Membrane-bound pyrophosphatases (M-PPases) are enzymes that couple the synthesis or hydrolysis of pyrophosphate (PPi) to the vectorial transport of protons and/or sodium ions. In addition, M-PPases can be divided into seven functional classes on the basis of their monovalent cation binding (K+-dependent and K+-independent enzymes) and pumping specificity (H+-pumps (H+-PPases), Na+-pumps (Na+-PPases) and H+ and Na+ co-pumps (Na+/H+-PPases)) and on the placement of a ‘semi-conserved glutamate' essential for pumping activity. So far, the structures of two M-PPases have been solved in three different states: TmPPase in resting and product-bound states (TmPPase:Ca:Mg and TmPPase:Pi2, respectively)11 and VrPPase in a substrate-analogue imidodiphosphate (IDP)-bound state (VrPPase:IDP)12. These structures have shown that M-PPases are homodimers, with each protomer having 16 transmembrane helices (TMHs) and a vertically arranged, continuous active site structure with four distinctive parts: ‘hydrolytic centre', ‘coupling funnel', ‘ion gate' and ‘exit channel'3. In this article we present three structures: the Na+-pumping TmPPase with IDP and Na+ bound (TmPPase:IDP) at 3.5 Å resolution, the H+-pumping VrPPase with one phosphate bound (VrPPase:Pi) at 3.5 Å resolution, and the newly refined structure of TmPPase with the phosphate analogue, WO4 bound, at 4 Å resolution (TmPPase:WO4).

In TmPPase:IDP, an Mg5IDP-complex was fit into the positive Fo–Fc density in the hydrolytic centre and then refined. The coordination of Mg2+ and IDP is almost identical to that seen in VrPPase:IDP12, even though the two enzymes pump different ions. Positive Fo–Fc density was seen in TmPPase:IDP between residues D6.50, E6.53, S6.54 and D16.46. A sodium ion was therefore refined into this density. The resulting bond distances were between 2.39–2.49 Å (mean: 2.43 Å) and the site was penta-coordinated (by the carboxylate groups of D6.50, E6.53 and D16.46, the Oγ of S6.54 and the main-chain carbonyl of D6.50)18. All of these results indicate that the density is most likely a bound Na+ and not a water molecule. Close to this, K16.50, which forms an ion-triplet in the resting-state TmPPase structure with D6.50 and E6.53, adopts a different orientation and the K16.50 Nζ is disordered. In TmPPase, sodium binding is facilitated by the inward motion of D16.46 into the sodium-binding site and by the movement of TMHs 6 and 16, which is almost twice as big as that in VrPPase. These helical movements bring D6.50, E6.53 and S6.54 to the correct position to bind Na+ and move K16.50 away from the binding site.

>MRGSHHHHHHYVAALFFLIPLVALGFAAANFAAVVRKPEGTERMKEISSYIRSGADSFLAHETKAIFKVAIVIAILLMIFTTWQTGVAFLLGAVMSASAGIVGMKMATRANVRVAEAARTTKKIGPALKVAYQGGSVMGLSVGGFALLGLVLVYLIFGKWMGQVDNLNIYTNWLGINFVPFAMTVSGYALGCSIIAMFDRVGGGVYTKAADMAADLVGKTELNLPEDDPRNPATIADNVGDNVGDVAGLGADLLESFVGAIVSSIILASYMFPIYVQKIGENLVHQVPKETIQALISYPIFFALVGLGCSMLGILYVIVKKPSDNPQRELNISLWTSALLTVVLTAFLTYFYLKDLQGLDVLGFRFGAISPWFSAIIGIFSGILIGFWAEYYTSYRYKPTQFLGKSSIEGTGMVISNGLSLGMKSVFPPTLTLVLGILFADYFAGLYGVAIAALGMLSFVATSVSVDSYGPIADNAGGISEMCELDPEVRKITDHLDAVGNTTAAIGKGFAIGSAIFAALSLFASYMFSQISPSDIGKPPSLVLLLNMLDARVIAGALLGAAITYYFSGYLISAVTKAAMKMVDEIRRQAREIPGLLEGKAKPDYNRCIEITSDNALKQMGYPAFIAILTPLVTGFLLGAEFVGGVLIGTVLSGAMLAILTANSGGAWDNAKKYLEAGNLEGYGKGSEPHKALVIGDTVGDPLKDTVGPSLDILIKIMSVVSVIAVSIFKHVHLF[2x]> SNARKIKTEPKQMHEDYCFQCGDGGELVMCDKKDCPKAYHLLCLNLTQP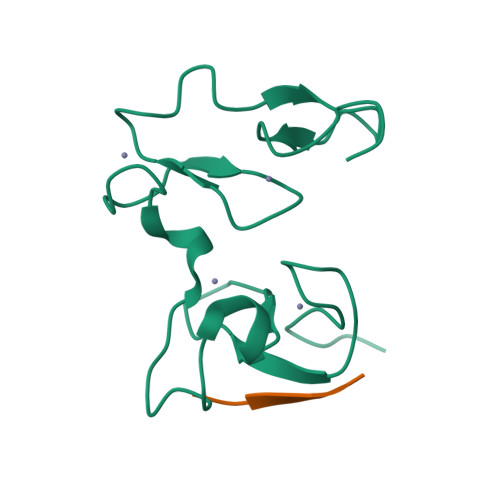PYGKWECPWHQCDECSSAAVSFCEFCPHSFCKDHEKGALVPSALEGRLCCSEHDPMAP;> ARTKQTA>SNAEKWTSTAIITQPDVGQIAGYNNAMNVIYGQAAPKVSDLQETLIGRFSSAFSALPETLDNQEEPEKLTIEPSVKNQQLPLTVSYVGQTAEGAQMKLAQYIQQVDDKVNQELEKDLKDNIALGRKNLQDSLRTQEVVAQEQKDLRIRQIQEALQYANQAQVTKPQVQQTEDVTQDTLFLLGSEALESMIKHEATRPLVFSPNYYQTRQNLLDIEKLKFDDLDIHAYRYVMKPTLPIRRDSPK[3x]

The Oag polymer chains are neither all of the same length nor of random length, and fall in a defined range termed the modal distribution. This distribution is regulated by two Wzz proteins in S. flexneri: WzzBSF, which confers an average modal chain-length of 10–17 Oag repeat units (short (S)-type), and WzzpHS2, which confers a very long (VL-type) modal chain-length of > 90 Oag repeat units. The S. flexneri Wzz proteins are members of the PCP1a family and are located in the inner membrane. They contain a hydrophilic periplasmic polypeptide segment, and two trans-membrane (TM) regions at the N- and C-terminal ends.

Site-directed and in-frame insertion mutagenesis studies of WzzBSF revealed that mutations in the TM or periplasmic regions can influence the Oag modal chain-lengths. Some WzzBSF mutants display shortened or lengthened Oag modal chain-length distribution, while other mutants display no change in Oag modal chain-length distribution or completely inactivate WzzBSF. The residue 107 is located in a helix in the base-domain of the protein, close to the trans-membrane regions. A107P confers a shortened Oag chain-length to bacteria and leads to a loss of resistance to colicin E2. Binding analyses reveal positive cooperativity for the interaction of very-short (VS) core-plus-Oag polysaccharide (COPS) with the periplasmic domain of WzzBSF, and a decreased COPS-binding affinity for the A107P mutant. The crystal structure of the mutant protein shows only subtle structural differences near the mutation, compared to the wild-type protein. Our observations suggest that a single amino-acid substitution on the inner surface of the periplasmic domain can lead to significant effects on the regulation on Oag modal chain-length, and implicates the LPS-binding affinity as an important parameter in the mechanism of this process.> MGGSHHHHHHGTMKQLISLK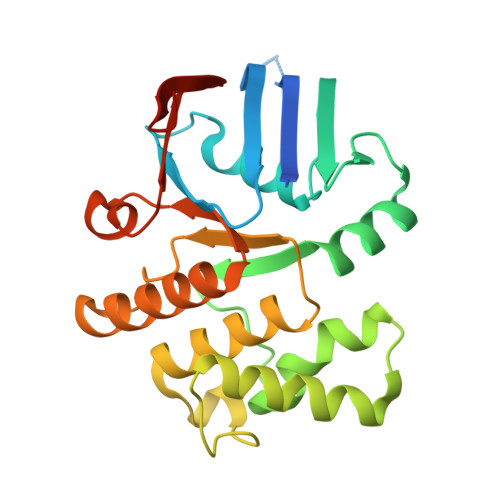NIFRSYRNGDQELQVLKNINLEVNEGEFVAIMGPSGSGKSTLMNTIGMLDTPTSGEYYLEGQEVAGLGEKQLAKVRNQQIGFVFQQFFLLSKLNALQNVELPLIYAGVSSSKRRKLAEEYLDKVELTERSHHLPSELSGGQKQRVAIARALVNNPSIILADEPTGALDTKTGNQIMQLLVDLNKEGKTIIMVTHEPEIAAYAKRQIVIRDGVISSDSAQLGKEEN Pseudomonas aeruginosa is a major gram-negative pathogen responsible for a variety of infections and possessing an array of both intrinsic and acquired resistance mechanisms, including β-lactamases, like the chromosomal Pseudomonas-derived cephalosporinase (PDC). β-Lactams are the most widely prescribed class of antibiotics in the United States, and antipseudomonal cephalosporins (including cefepime) are important therapies (alone or combined with β-lactamase inhibitors) for P. aeruginosa infections. Taniborbactam (formerly VNRX-5133) is a novel, investigational, bicyclic boronate β-lactamase inhibitor shown to inhibit members of all four Ambler classes of β-lactamase enzymes. PDC-88 was chosen as a representative member of the group for detailed characterization and is noted for a T289-P290 deletion (by structural alignment-based numbering of class C β-lactamases, “SANC”) in the R2-loop (ΔT289-P290). Herein, we focus our efforts on PDC-88 to better understand both the basis of this expanded-spectrum activity and its inhibition by taniborbactam.

The active sites of the PDC-3 and PDC-88 structures in complex with taniborbactam revealed strong electron density for the bicyclic boronic acid inhibitor. Taniborbactam was covalently bonded to the hydroxyl group of the PDC catalytic serine (S64 by SANC) and made extensive interactions in both the PDC-3 and PDC-88 active sites. The boron ring oxygen hydrogen bonded with the side chain of Y150. The cyclohexane ring of taniborbactam made van der Waals interactions with Y221. A minor difference between the taniborbactam binding modes in PDC-3 and PDC-88 was that residue Q120 in the latter hydrogen bonded with the amide oxygen (3.1 Å distance) of taniborbactam, whereas PDC-3 did not (distance is larger in PDC-3 at 3.6 Å). Superimposing the taniborbactam-bound PDC-3 and PDC-88 structures onto their respective apo structures indicated that binding of the inhibitor caused only minor conformational changes. For PDC-88, in addition to the Y150 change as observed for PDC-3, residue Q120 moved toward the active site to make a hydrogen bond with the amide moiety of taniborbactam. Also, upon binding of taniborbactam, L293 shifted toward the inhibitor to facilitate a 4.8 Å hydrophobic/van der Waals interaction with the bicyclic ring scaffold of taniborbactam. The similar binding mode and interactions for taniborbactam in PDC-3 and PDC-88 agree with the similar Ki app values measured for the inhibitor.

> DEAPADRLKALVDAAVQPVMKANDIPGLAVAISLKGEPHYFSYGLASKEDGRRVTPETLFEIGSVSKTFTATLAGYALAQDKMRLDDRASQHWPALQGSRFDGISLLDLATYTAGGLPLQFPDSVQKDQAQIRDYYRQWQPTYAPGSQRLYSNPSIGLFGYLAARSLGQPFERLMEQQLFPALGLEQTHLDVPEAALAQYAQGYGKDDRPLRVGPGPLDAEGYGVKTSAADLLRFVDANLHPERLDRPWAQALDATHRGYYKVGDMTQGLGWEAYDWPISLKRLQAGNSMALQPHRIARLPAPQALEGQRLLNKTGSTNGFGAYVAFIPGRDLGLVILANRNYPNAERVKIAYAILSGLEQQAKVPLKR> MALGPFVLPFRGDQYSFGINFKSSPEEKLNFDLSCVAFDVKGQLHDTLHARKPTALDGALVKGFEKQALPEETVQVEGDDVIYMFPKKFERQVEVLLFVASAPSIPGKKHDLDSSSKLEFAVSYSDVGGQAFNQSFDLKPLAAQGGVSSIIVAVMYLQAEGGWTLRSVGDCHPFDSPGLIVPELKQTILNLRDHHGVQLDAADAIQAIDPAERVPVTRQFQDQSLDEASAGRAAEPAPVKKLRIDLSWTFWPPPPPTEEGEEPPEEPALEYNLVMYNKDGEEVQSISTGNREATGARAGRPEPEEDEEEEKEEEKEEPEEGEEGEEGEGGEPKEPPPPPPAPKVDPYEFKERDVIYLDVPDLPAEVRSMVLLVTNYDEENGFTRVRTVRCRLVDVSNGEAPLPGSKAAVAAAAAAAEQGLAAPPNPERVLADYGVLSKYEDDKATTQVALMKLYKEYA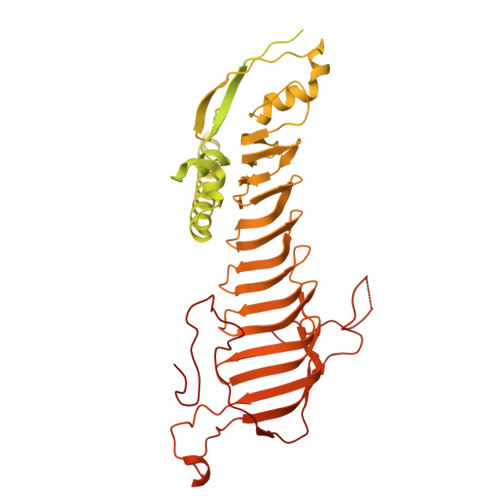DSAFNVFRGAGVDNVAAFIGQEPDTIINQLKAYLEATKKQKAAEAAAAAAAEESGEEITADPKPHVWRFRALGLNFGGDSLEAIEHDLKNLFAFDGDLAPGAARDSDTSRSSFPNGDTYFGSYADDVKHGPGLYAFATGAGYAGEYAGGKRHGRGVMVFPDGGTYVGEFVADKFEGQGQYRYPDGSVYTGSWAAGQKHGPGVYWDTARGCLRGEWKKGLLVGKGTYEQPALRFEGEFVRGMPAGTATYTLTGHRTLDMPCFAAQHIQAEEGPTLALPCAYGIPPGSGDEPQLDEEGQPIEDTDKPPLPAHPKYEGLTFTAEQLPGAAPDTVFPPEEGKPVPITAVPAFSVSTGLVA>MFQQLSARLQEAIGRLRGRGRITEEDLKATLREIRRALMDADVNLEVTRDFVERVREEALGKQVLESLTPAEVILATVYEALKEALGGEARLPVLKDRNLWFLVGLQGSGKTTTAAKLALYYKGKGRRPLLVAADTQRPAAREQLRLLGEKVGVPVLEVMDGESPESIRRRVEEK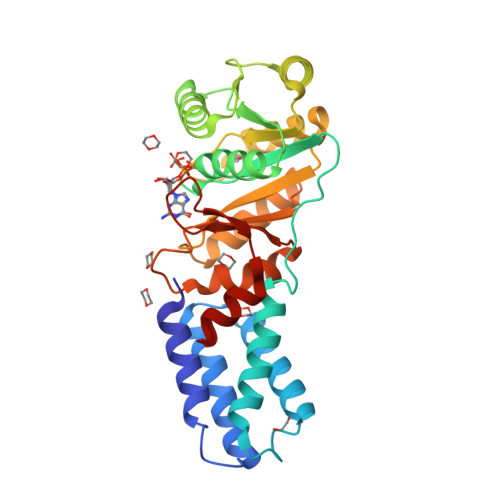ARLEARDLILVDTAGRLQIDEPLMGELARLKEVLGPDEVLLVLDAMTGQEALSVARAFDEKVGVTGLVLTKLDGDARGGAALSARHVTGKPIYFAGVSEKPEGLEPFYPERLAGRILGMGDV[2x]> 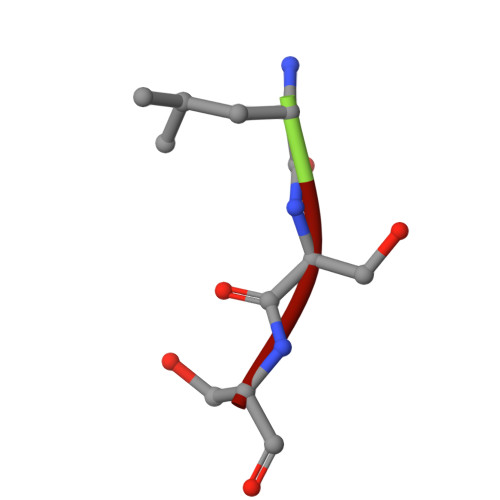LSS>[2x]EKPADSGPAVAQNTEYVGDEACKTCHSDVHSAWSETSHGNFIKDVTKDPKALPGNFEGNYPKMLNFKAEDIQYVLLGKPGALKVQELVGKKGTFGVPADDYPVMWASWDAGKGEWEIEVEAIGEGTPWLSTCAGCHVTGLTVPTDKNPKAAKAFAGFGITCEQCHGPGAKHIKNPQGEKMVISYDAENCGQCHSRGDSVAKTPDGKPFGYPYNDEGQYVPGKKLADYYTVVSVEGDKEGKLFWPTKHAKNSHHLQYP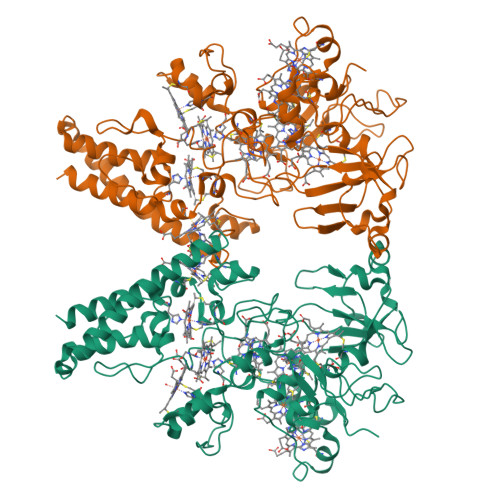EWLMTGHATALETLKGNGHAQDRCLKCHSAEAYLAKEGTTVTMNDAKLGVTCQVCHASHDPAATKEAFLRKPKTEICTQCHNAEGGIVAGKEVHHPHKEMNEGKIGLGFPDSPSVMYKAGVTCVDCHMPKTAGPKASHLMKVVMPKDGKANGMPDSCSSCHPGASQDYLQNVIDTWQNDIKGRLAKVKAKLDAKKAAANSQAYKEALTYYSIVAADGSNGVHNYDLAVKLLTAAEQKLQKGELKLEGKPIPDPLLGLDSTRTGHHHHHH>[2x]GDPAERTWIFSGAELKQAIEGKLAPDVSDPEMRRLVSVAKSSAYIAGVADLTSGSDWCGAGAVAPHELTDRIYTYLGDMPAEKLDEQAATLVREALKVSFPCEQKSN;>[2x]MMRVNFDTLYSNYPSSDPSHPNYLSQRDLFTEIGWESFIGNPNYHNTCAIRVSIAFVKSGINIVPSSHRIQKGPYAGKGIEVNMRRLATLMKRTSYLGEPDPYTPATARNGIGARNGVVAFNNIPGYTGGGHIDLVRGGSEATQCASACYYNSETIWFWPLQAS

The type VI secretion systems (T6SSs) of Gram-negative bacteria inject various toxic effectors into the periplasmic or cytoplasmic space of the target cells and induce cell lysis of enemy cells. The various T6SS-related amidase effector proteins (Taes) are classified into four families (Tae1, Tae2, Tae3 and Tae4) based on their cleavage specificities. Tai1, Tai2, Tai3 and Tai4 neutralize the endogenous toxic effectors Tae1, Tae2, Tae3 and Tae4, respectively. To gain insight into the Tae4 family proteins, we determined the crystal structures of Tai4 and of the Tae4–Tai4 complex from Agrobacterium tumefaciens at 1.55 and 1.9 Å resolution, respectively.

The structure revealed that the AtTai4 dimer binds two AtTae4 molecules to form a heterotetramer in the asymmetric unit, which is consistent with the size-exclusion chromatography results indicating that the AtTae4–AtTai4 complex exists in a heterotetrameric form in solution. Pro47, Asp48 and Val49 in the loop of AtTai4 form hydrogen bonds to Arg108, Thr142 and Arg108 in the other AtTae4 protomer in the asymmetric unit, respectively. Thus, these specific interactions between AtTae4 and AtTai4 may contribute towards stabilizing the formation of the AtTae4–AtTai4 complex. Comparisons of these structures with those of homologous proteins revealed that the AtTae4–AtTai4 complex shares structural similarity with the SmTae4–SmTai4 complex. A structural comparison of AtTai4 with SmTai4 showed that AtTai4 contains more extended helices and loops, which may enforce the interaction between AtTai4 and the adjacent AtTae4. While there is no direct interaction between the potentially catalytic His131 of AtTae4 and Ala86 of AtTai4, which corresponds to Gln84 of SmTai4, the structural comparison suggests that AtTai4 effectively neutralizes the activity of AtTae4 by blocking the entrance to its substrate-binding pocket. The growth inhibition of E. coli DH10B owing to the expression of AtTae4 was rescued by the co-expression of AtTai4. The Tae4 family proteins have conserved catalytic residues (Cys–His–Asp) that are responsible for their peptidoglycan amidase activity. A structural superimposition highlighted the differences in the spatial arrangement of the aspartic acid residue in the catalytic triad (Cys–His–Asp) among the Tae4 family proteins. Thus, the present structure re­inforces the idea that the Tae4 family proteins have two types of structurally distinct catalytic triads.> GPHMLEMPKEKYEPPDPRRMYTIMSSEEAANGKKSHWAELEISGKVRSLSASLWSLTHLTALHLSDNSLSRIPSDIAKLHNLVYLDLSSNKIRSLPAELGNMVSLRELHLNNNLLRVLPFELGKLFQLQTLGLKGNPLTQDILNLYQEPDGTRRLLNYLLDNLSGTAKRITTEQPPPRSWIMLQEPDRTRPTALFSVMCYNVLCDKYATRQLYGYCPSWALNWDYRKKAIIQEILSCNADIVSLQEVETEQYYSFFLVELKERGYNGFFSPKSRARTMSEQERKHVDGCAIFFKTEKFTLVQKHTVEFNQLAMANSEGSEAMLNRVMTKDNIGVAVLLELRKESIEMPSGKPHLGTEKQLILVANAHMHWDPEYSDVKLVQTMMFLSEVKNIIDKASRNLKSSVLGEFGTIPLVLCADLNSLPDSGVVEYLSTGGVETNHKDFKELRYNESLTNFSCHGKNGTTNGRITHGFKLQSAYESGLMPYTNYTFDFKGIIDYIFYSKPQLNTLGILGPLDHHWLVENNISGCPHPLIPSDHFSLFAQLELLLPFLPQVNGIHLPGRR;> GPHMLEPAATVDHSQRICEVWACNLDEEMKKIRQVIRKYNYVAMDTEFPGVVARPIGEFRSNADYQYQLLRCNVDLLKIIQLGLTFMNEQGEYPPGTSTWQFNFKFNLTEDMYAQDSIELLTTSGIQFKKHEEEGIETQYFAELLMTSGVVLCEGVKWLSFH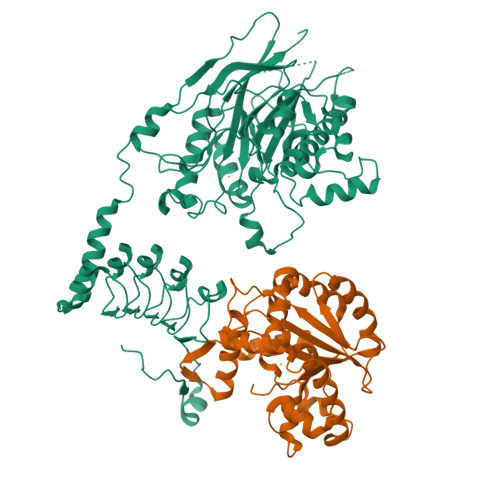SGYDFGYLIKILTNSNLPEEELDFFEILRLFFPVIYDVKYLMKSCKNLKGGLQEVAEQLELERIGPQHQAGSDSLLTGMAFFKMREMFFEDHIDDAKYCGHLYGLGSGSSYVQNGTGNAYEEEANKQS>[2x]MAGNKKINRREEILQALAEMLESNEGASRITTAKLAKQVGVSEAALYRHFPSKTRMFEGLIEFIEESLMSRINRIFDEEKDTLNRIRLVM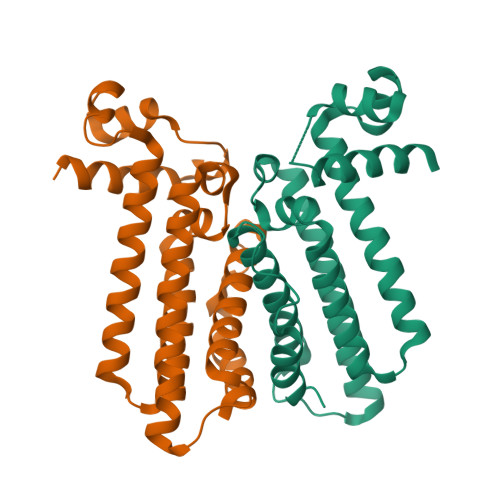QLLLAFAERNPGLTRILSGHALMFENERLRDRINQLFERIETSLRQILRERKLREGKSFPVDENILAAQLLGQVEGSLNRFVRSDFKYLPTANFDEYWALLSAQIK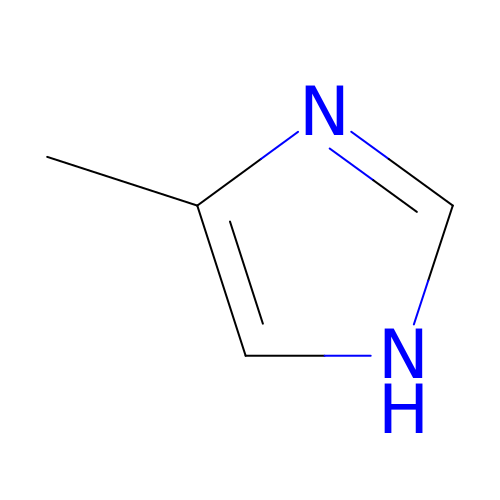4-METHYLIMIDAZOLE | C4 H6 N2 | XLSZMDLNRCVEIJ-UHFFFAOYSA-N> MRNELEEMQRRADQLADESLEST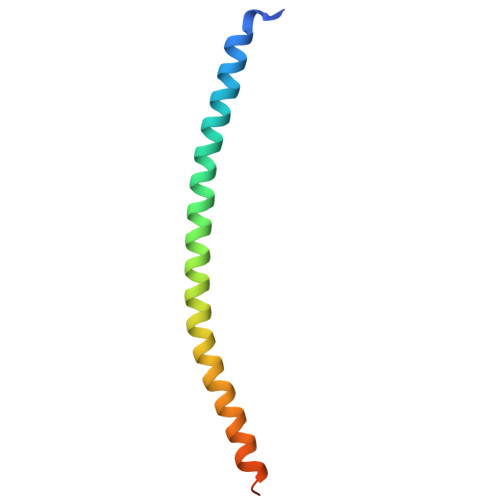RRMLQLVEESKDAGIRTLVMLDEQGEQLDRVEEGMNHINQDMKEAEKNLKDLGK>GPGSSGPADCCRMKECCTDRVNECLQRYSGREDKFVSFCYQEATVTCGSFNEIVGCCYGYQMCM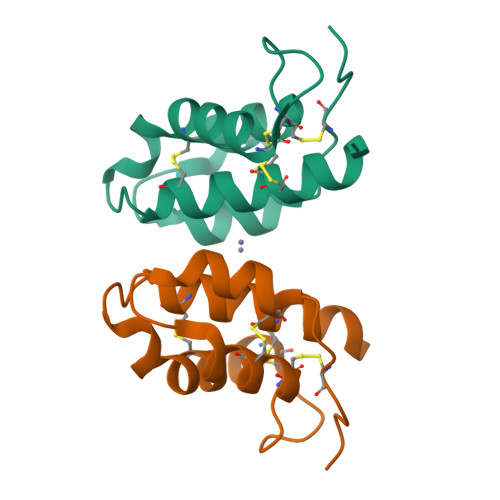IRVVKPNSLSGAHEACKTVSCGNPCA[2x]> SLLISYESDFKTTLEQAKASLAEAPSQPLSQRNTTLKHVEQQ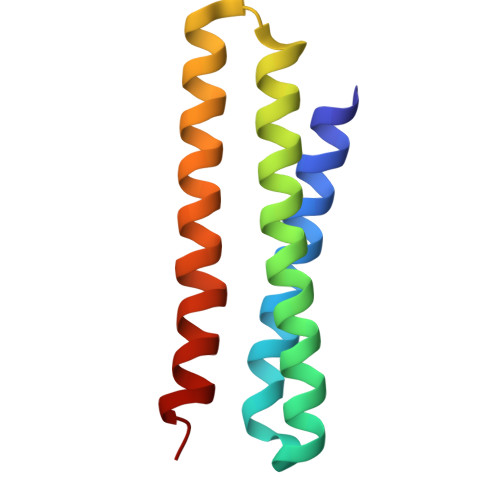QDELFDLLDQMDVEVNNSIGDASERATYKAKLREWKKTIQSDIKRPLQSLVDSGD2-((1-(but-2-yn-1-yl)-1H-pyrazol-4-yl)(cyclopropylmethyl)amino)-5-(4-(dimethylcarbamoyl)-1H-pyrrol-2-yl)thiazole-4-carboxamide | C22 H25 N7 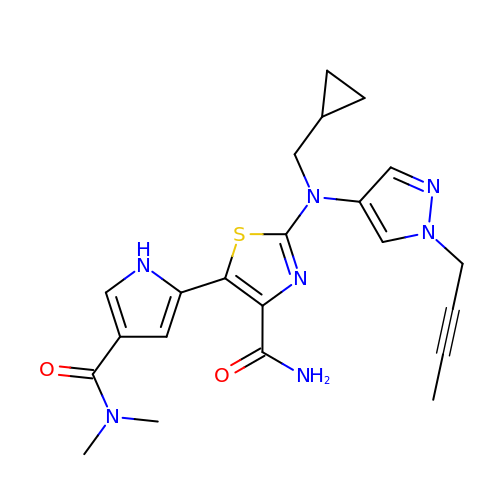O2 S | HACYEVIDLDLIII-UHFFFAOYSA-N>[3x]XGELKAIAQ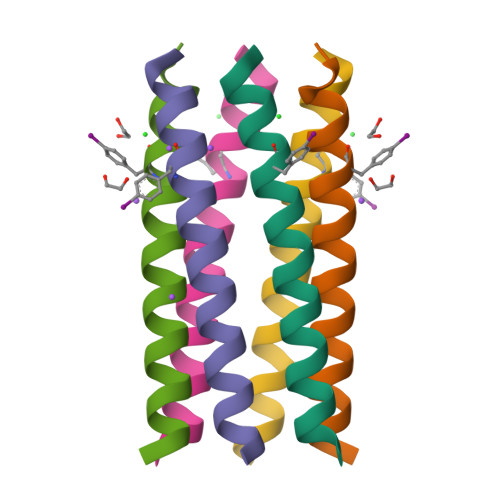ELKAIAKELKAIAFELKAIAQGAGX>[2x]DIVSEKKPATEVDPTHFEKRFLKRIRDLGEGHFGKVELCRYDPE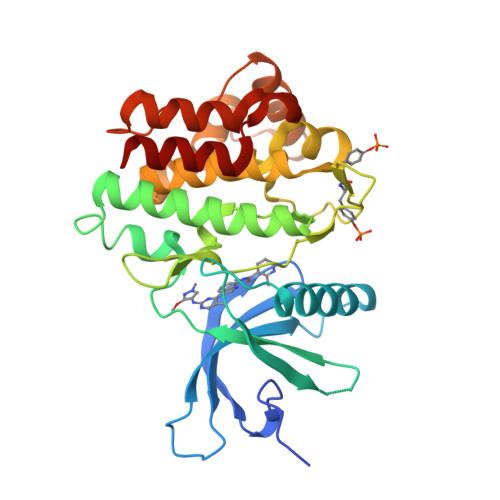GDNTGEQVAVKSLKPESGGNHIADLKKEIEILRNLYHENIVKYKGICTEDGGNGIKLIMEFLPSGSLKEYLPKNKNKINLKQQLKYAVQICKGMDYLGSRQYVHRDLAARNVLVESEHQVKIGDFGLTKAIETDKEYYTVKDDRDSPVFWYAPECLMQSKFYIASDVWSFGVTLHELLTYCDSDSSPMALFLKMIGPTHGQMTVTRLVNTLKEGKRLPCPPNCPDEVYQLMRKCWEFQPSNRTSFQNLIEGFEALLK> MTDALEQSV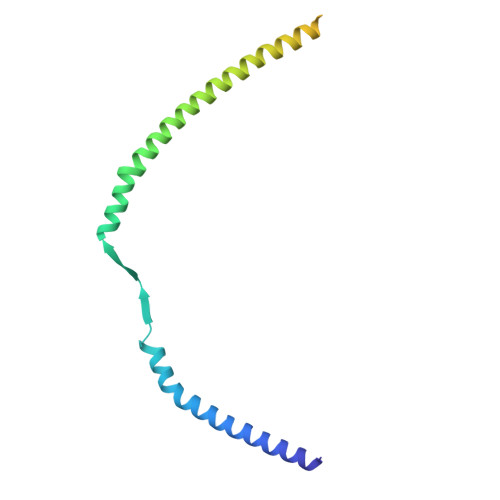LALEGTVSVLKDSVESLKCANEPSTNLASTMLQTKRVFRLVPEYDVERSKLDLIEEVEPLVRTLGDKLRKSMGRMQRELDTLQQTYELNDLRLKKNISMDDDDALNSPDMGQEYEGRDADDVVMMASSTNEELEELKKLKEKKKQLENKLEILKQK>[2x]MDASLTGAVAELGTSKAAARIRAAAI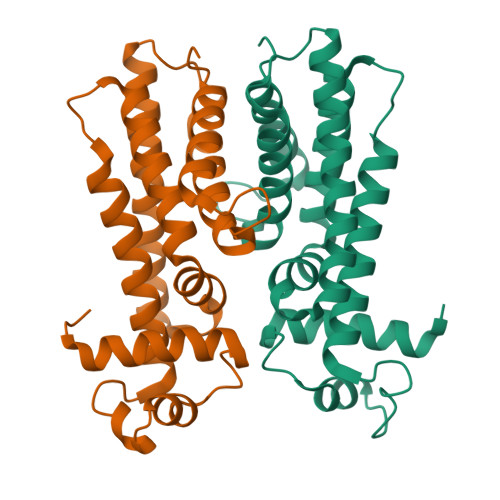EVFAAKGYGATTTREIAASLDMSPGAVYPHYKTKESLLYAISLEGHHSVLAAITAADFPDIAAPDRLMSTVTAYVTWHADNRASARVGQYELRSLSPEHFAIIADIRRSTTKVFTRIIEAGATAGDFHPFDIEAAALAITSLGIDVSRWFPSHTYSDPRIIAARYVELALRMVGCADRQPLDKPS L-gamma-glutamyl-S-[(3S)-1-ethyl-2,5-dioxopyrrolidin-3-yl]-L-cysteinylglycine | C16 H24 N4 O8 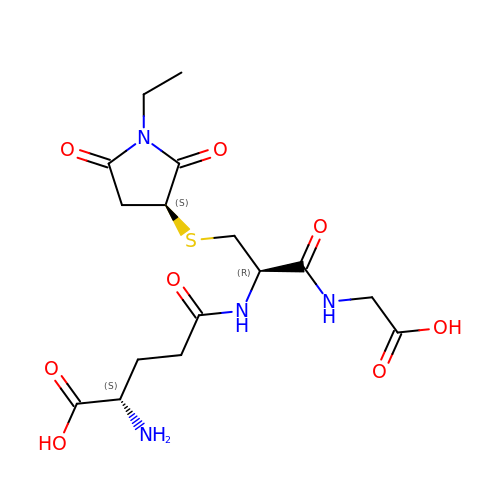S | QCPAUAAIPLHRLB-GUBZILKMSA-N>KPKLLNKFDKTIKAELDAAEKLRKRGKIEEAVNAFKELVRKYPQSPRARYGKAQCEDDLAEKRRSNEVLRGAIETYQEVASLPDVPADLLKLSLKRRSDRQQFLGHMRGSLLTLQRLVQLFPNDTSLKNDLGVGYLLIGDNDNAKKVYEEVLSVTPNDGFAKVHYGFILKAQNKIAESIPYLKEGIESGDPGTDDGRFYFHLGDAMQRVGNKEAYKWYELGHKRGHFASVWQRSLYNVNGLKAQPWWTPKETGYTELVKSLERNWKLIRDEGLAVMDKAKGLFLPEDENLREKGDWSQFTLWQQGRRNENACKGAPKTCTLLEKFPETTGCRRGQIKYSIMHPGTHVWPHTGPTNCRLRMHLGLVIPKEGCKIRCANETKTWEEGKVLIFDDSFEHEVWQDASSFRLIFIVDVWHPELTPQQRRSLPAI[2x];> AKDGLGEYTCTSLEG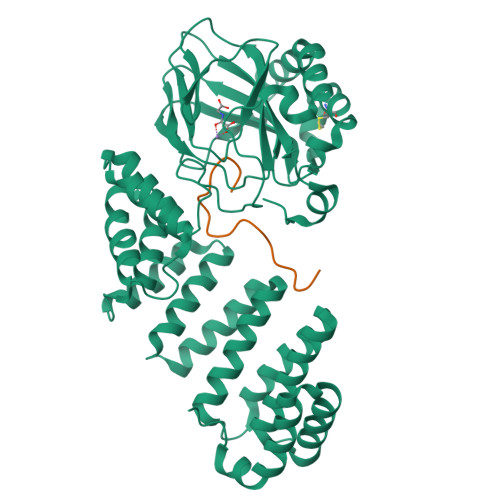FEGK>[2x]GSHMATPWSGYLDDVSAKFDTGV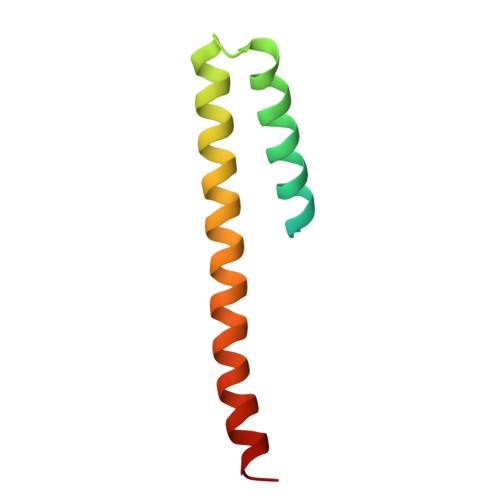DNLQTQVTEALDKLAAKPSDPALLAAYQSKLSEYNLYRNAQSNTAKAFKDIDAAIIQNFR>[2x]QTASPVIPTDPAIETHIREWLQKMTLEQKIGQMCEITIDVVSDLETSRKKGFCLSEAMLDTVIGKYKVGSLLNVPLGVAQKKEKWAEAIKQIQEKSMKEIGIPCIYGVDQIHGTTYTLDGTMFPQGINMGATFNRELTRRGAKISAYETKAGCIPWTFAPVVDLGRDPRWARMWENYGEDCYVNAEMGVSAVKGFQGEDPNRIGEYNVAACMKHYMGYGVPVSGKDRTPSSISRSDMREKHFAPFLAAVRQGALSVMVNSGVDNGLPFHANRELLTEWLKEDLNWDGLIVTDWADINNLCTRDHIAATKKEAVKIVINAGIDMSMVPYEVSFCDYLKELVEEGEVSMERIDDAVARVLRLKYRLGLFDHPYWDIKKYDKFGSKEFAAVALQAAEESEVLLKNDGNILPIAKGKKILLTGPNANSMRCLNGGWSYSWQGHVADEYAQAYHTIYEALCEKYGKENIIYEPGVTYASYKNDNWWEENKPETEKPVAAAAQADIIITCIGENSYCETPGNLTDLTLSENQRNLVKALAATGKPIVLVLNQGRPRIINDIVPLAKAVVNIMLPSNYGGDALANLLAGDANFSGKMPFTYPRLINALATYDYKPCENMGQMGGNYNYDSVMDIQWPFGFGLSYTNYKYSNLKVNKPTFNADDELIFTVDVTNTGKVAGKESVLLFSKDLVASSTPDNIRLRNFEKVSLEPGETKTVTLKLKGSDLAFVGYDGKWRLEKGDFKIKCGDQWMDIVCDQTKVWNTPNKNTLHKLEHHHHHH

In this context, we recently reported the characterization of a novel xyloglucan utilization locus (XyGUL) that confers Bacteroides ovatus, and species harbouring syntenic XyGULs, with the ability to utilize this abundant vegetable polysaccharide across sampled human populations. Here, we present the three-dimensional structures of BoGH31, BoGH43A, BoGH43B and BoGH3B, expanding our knowledge of the structural determinants required for xyloglucan degradation. Our analyses highlight key adaptations in these enzymes that confer their specificity for xyloglucan oligosaccharides, while also providing a rationale for the maintenance of two divergent genes coding for GH3 enzymes, and similarly two divergent genes for GH43 family members, within the same PUL. While we were unable to determine a structure for BoGH3A, our structural and sequence analysis of BoGH3B has also allowed us to highlight further potential differences between these two enzymes encoded by the operon. Together with existing biochemical data, our analyses of the three-dimensional structures, and various enzyme-inhibitor complexes, of BoGH31, BoGH43A, BoGH43B and BoGH3B provide molecular-level insight into the stepwise breakdown of xyloglucan by the BoXyGUL.

Like GH43, there are two GH3 members (BoGH3A and BoGH3B) present in the Bo XyGUL, both of which have been shown to be β-glucosidases with very similar specific activities. BoGH3B comprises a three-domain architecture, consisting of an N-terminal (TIM) barrel-like domain (residues 26 to 419), a central α/β sandwich domain (residues 420 to 660) and a fibronectin type-III (FN-III)-like domain at the C-terminus (residues 661–782). The dimeric organization of this novel enzyme appears potentially important for function, with a large, flexible loop reaching over from one protomer to contact the substrate and fully assemble the active site of the neighbouring molecule. BoGH3B was found to co-purify with glucose in its active site. This could readily be modelled with a 4C1 chair conformation, highlighting the position of the −1 sub-site. Within the GH3B active site, putative catalytic nucleophile (Asp314) and acid/base (Glu534) residues can be observed in close proximity to the glucose moiety, poised for nucleophilic attack. Away from the −1 sub-site, the exterior surface structure of the GH3B active pocket deviates from the most closely related homologues, presenting as a more closed structure similar to that seen in the distantly related barley β-glucosidase. GH3B has significant activity for glucose-only oligosaccharides but displays far weaker activity on xyloglucan-derived oligos, which retain their xylose side chains. Similar to barley β-glucosidase, such observations might suggest that the narrowing of the active site cleft could be responsible for the high specificity of BoGH3B towards β-1,4-linked glucans.>GSGEIRPTIGQQMETGDQRFGDLVFRQLAPNVWQHTSYLDMPGFGAVASNGLIVRDGGRVLVVDTAWTDDQTAQILNWIKQEINLPVALAVVTHAHQDKMGGMDALHAAGIATYANALSNQLAPQEGMVAAQHSLTFAANGWVEPATAPNFGPLKVFYPGPGHTSDNITVGIDGTDIAFGGCLIKDSKAKSLGNLGDADTEHYAASARAFGAAFP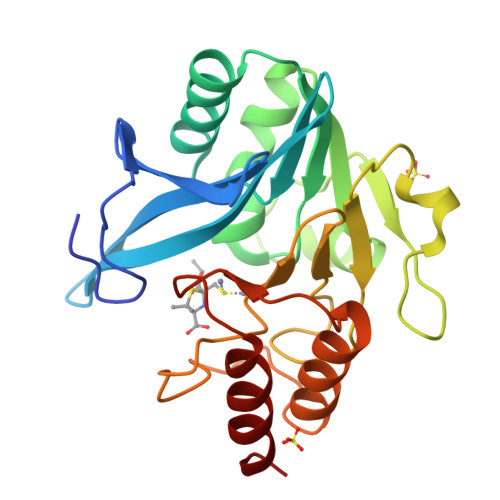KASMIVMSHSAPDSRAAITHTARMADKLR[2x]>[2x]GADDVVDSSKSFVMENFSSYHGTKPGYVDSIQKGIQKPKSGTQGNYDDDWKEFY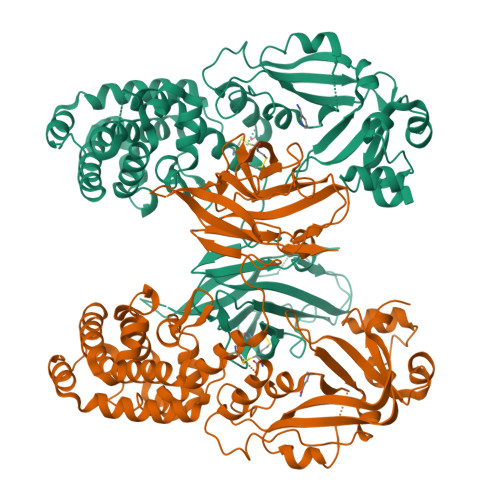STDNKYDAAGYSVDNENPLSGKAGGVVKVTYPGLTKVLALKVDNAETIKKELGLSLTEPLMEQVGTEEFIKRFGDGASRVVLSLPFAEGSSSVEYINNWEQAKALSVELEINFETRGKRGQDAMYEYMAQACAGNRVRRSVGSSLSCINLDWDVIRDKTKTKIESLKEHGPIKNKMSESPNKTVSEEKAKQYLEEFHQTALEHPELSELKTVTGTNPVFAGANYAAWAVNVAQVIDSETADNLEKTTAALSILPGIGSVMGIADGAVHHNTEEIVAQSIALSSLMVAQAIPLVGELVDIGFAAYNFVESIINLFQVVHNSYNRPAYSPGHKTQPFLHDGYAVSWNTVEDSIIRTGFQGESGHDIKITAENTPLPIAGVLLPTIPGKLDVNKSKTHISVNGRKIRMRCRAIDGDVTFCRPKSPVYVGNGVHANLHVAFHRSSSEKIHSNEISSDSIGVLGYQKTVDHTKVNSKLSLFFEIKS> APAVADKADNAFMMICTALVLFMTIPGIALFYGGLIRGKNVLSMLTQVTVTFALVCILWVVYGYSLAFGEGNNFFGNINWLMLKNIELTAVMGSIYQYIHVAFQGSAACITVGLIVGALAERIRFSAVLIFVVVWLTLSYIPIAHMVWGGGLLASHGALDFAGGTVVHINAAIAGLVGAYLIGKRVGFGKEAFKPHNLPMVFTGTAILYIGWFGFNAGSAGTANEIAALAFVNTVVATAAAILGWIFGEWALRGKPSLLGACSGAIAGLVGVTPACGYIGVGGALIIGVVAGLAGLWGVTMLKRLLRVDDPCDVFGVHGVCGIVGCIMTGIFAASSLGGVGFAEGVTMGH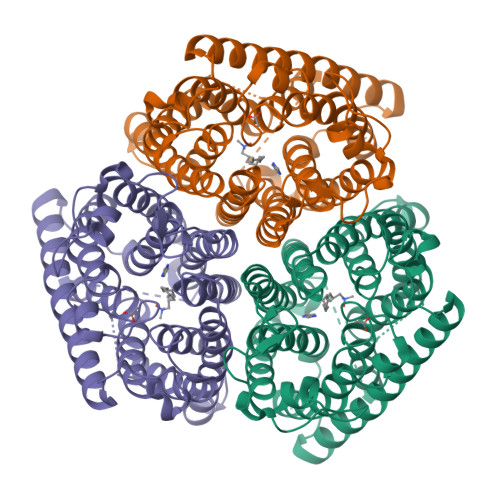QLLVQLESIAITIVWSGVVAFIGYKLADLTVGLRVPEEQEREGLDVNSHGENAYNADQAQQPAQADLEHHHHHH>[2x]MSRLDKSKVINSALELLNEVGIEGLTTRKLAQKLGVEQPTLYWHVKNKRALLDAL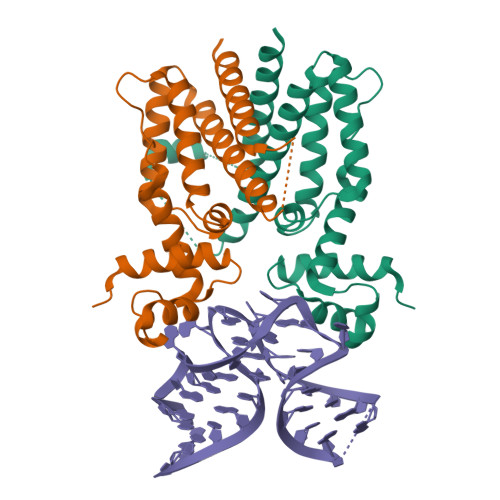AIEMLDRHHTHFSPLEGESWQDFLRNNAKSFRNALLSHRDGAKVHLGTRPTEKQYETLENQLAFLTQQGFSLENALYALSAVGHFTLGSVLEDQEHQVAKEERETPTTDSMPPLLRQAIELFDHQGAEPAFLHGLESLIRGFEVQLTALLQIV>DAAPGASKLRAVLEKLKLSRDDISTAAG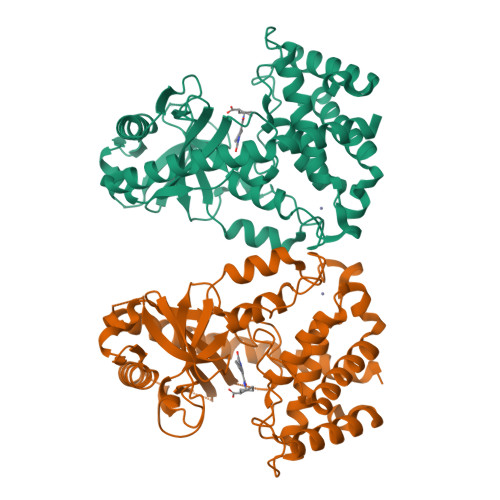MVKGVVDHLLLRLKCDSAFRGVGLLNTGSYYEHVKISAPNEFDVMFKLEVPRIQLEEYSNTRAYYFVKFKRNPKENPLSQFLEGEILSASKMLSKFRKIIKEEINDIKDTDVIMKRKRGGSPAVTLLISEKISVDITLALESKSSWPASTQEGLRIQNWLSAKVRKQLRLKPFYLVPKHAKEGNGFQEETWRLSFSHIEKEILNNHGKSKTCCENKEEKCCRKDCLKLMKYLLEQLKERFKDKKHLDKFSSYHVKTAFFHVCTQNPQDSQWDRKDLGLCFDNCVTYFLQCLRTEKLENYFIPEFNLFSSNLIDKRSKEFLTKQIEYERNNEFPVFDEF[2x]>MTTATAGLAVELKQSTAQAHEKAEHSTFMSDLLKGRLGVAEFTRLQEQAWLFYTALEQAVDAVRASGFAESLLDPALNRAEVLARDLDKLNGSSEWRSRITASPAVIDYVNRLEEIRDNVDGPALVAHHYVRYLGNLSGGQVIARMMQRHYGVDPEALGFYHFEGIAKLKVYKDEYREKLNNL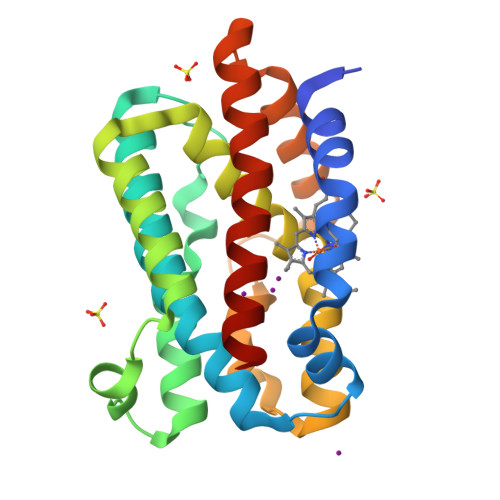ELSDEQREHLLKEATDAFVFNHQVFADLGKGL[3x]>DRHHHHHHKLQHAPPWTEDCRKSTYPPSGPTYRGAVPWYTINLDLPPYKRWHELMLDKAPMLKVIVNSLKNMINTFVPSGKVMQVVDEKLPGLLGNFPGPFEEEMKGIAAVTDIPLGEIISFNIFYELFTI[2x];>[2x]CTSIVAEDKKGHLIHGRNMDFGVFLGWNINNDTWVITEQLKPLTVNLDFQRNNKTVFKASSFAGYVGMLTGFKPGLFSLTLNERFSINGGYLGILEWILGKKDAMWIGFLTRTVLENSTSYEEAKNLLTKTKILAPAYFILGGNQSGEGCVITRDRKESLDVYELDAKQGRWYVVQTNYDRWKHPFFLDDRRTPAKMCLNR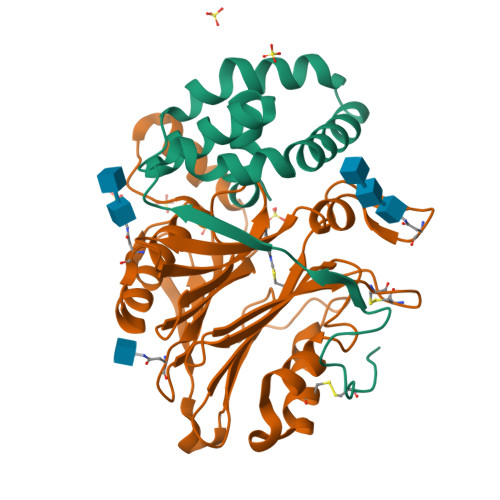TSQENISFETMYDVLSTKPVLNKLTVYTTLIDVTKGQFETYLRDCPDPCIGW Colonization factor antigen I (CFA/I) is a representative member of alternative chaperone-usher fimbriae in enterotoxigenic Escherichia coli, a major cause of travelers' diarrhea. For the CFA/I fimbriae, one subunit is the single-copy, tip-locating adhesin CfaE and the other is the major pilin CfaB, polymerizing to form the helical shaft of a CFA/I fimbria[4–6]. In addition to the two structural subunits, biogenesis of CFA/I fimbriae requires the functions of two factors, the periplasmic chaperone CfaA and the outer membrane usher protein CfaC, which bear functional similarities to components required for fimbriae that are assembled by “the chaperone-usher” (CU) pathway[11–19]. We demonstrate that the chaperone-tip adhesin complex CfaA-CfaE is essential in early fimbriae growth.

When compared to native CfaA, the mutant variant containing the triple residue substitution T112I/L114I/V116I on G1 strand (hitherto referred to as mtCfaA) formed significantly stabilized complexes with CfaE, CfaB and CfaBntd (the CfaB variant lacking the N-terminal donor strand). There are two identical copies of the mtCfaA-CfaE complex in one crystallographic asymmetric unit. The structure was refined to 2.77Å resolution with Rwork of 22.5% and Rfree of 26.0%. In the structural model of the complex, the loops containing residues 100–109 in mtCfaA and residues 311–320 in CfaE were not built because of poor electron density in those regions. CfaA interacts with CfaE in the canonical DSC manner via a pair of parallel β-strands: one from the CfaA G1 strand and the other from the CfaE F2 strand. Compared to the mtCfaA-CfaBntd structure, the mtCfaA-CfaE structure reveals a slightly more open cleft between the two domains of CfaA to accommodate the larger CfaE adhesin. The differences in hydrophobic side chains of these residues in CfaE, especially for the residues F353 (M130 in CfaB) at P0 and Y20 (L221 in CfaB) at P5, lead to a shallower, narrower groove for binding to the CfaA G1 strand, which is consistent with weaker interactions between the adhesin and chaperone. The main-chain and side-chain oxygen atoms of CfaE S357 form hydrogen bonds with the essential cleft residue pair N180’/Y182’ and the conserved residue E46’ (residues from CfaA are marked with’), while Q358, T359, and L360 interact with T43’, N180’, and N203’ through main-chain and side-chain hydrogen bonds. Nearby the adhesin subunit C-terminus, residue R253 of the C2’ strand of CfaE interacts with residues E48’ and Y92’ from CfaA, contributing to anchorage of the subunit to the cleft region. Upon binding to CfaA, the dscCfaE has its two domains re-arranged with the joint angle measured at 161.4°.

>[2x]ANFMIYPISKDLKNGNSELVRVYSKSKEIQYIKIYTKKIINPGTTEEYEVDIPNWDGGLVVTPQKVILPAGASKSIRLTQFKIPKKEEVYRVYFEAVKPDSKENVIDNKKLTIEISINIIYAALIRSLPSEQNISLNISRNAKKNIIIYNNGNVRAGVKDIYFCKSSNIDDNCVKKAYNKNIYPEKSFDTLVNNNFSYVFIKLNHEGIEKEQGLIQLKVPA;>[2x]HHHHDKNPGSENMTNTIGPHDRGGSSPIYNILNSYLTAYNGSHHLYDRMSFLCLSSQNTLNGACPSSDAPGTATIDGETNITLQFTEKRSLIKRELQIKGYKQFLFKNANCPSKLALNSSHFQCNREQASGATLSLYIPAGELNKLPFGGVWNAVLKLNVKRRYDTTYGTYTINITVNLTDKGNIQIWLPQFKSNARVDLNLRPTGGGTYIGRNSVDMCFYDGYSTNSSSLEIRFQDDNSKSDGKFYLKKINDDSKELVYTLSLLLAGKNLTPTNGQALNINTASLETNWNRITAVTMPEISVPVLCWPGRLQLDAKVKNPEAGQYMGNIKITFTPSSQTL> SADAQSFLNRVCGVSAARLTPCGTGTSTDVVYRAFDIYNDKVAGFAKFLKTNCCRFQEKDEDDNLIDSYFVVKRHTFSNYQHEETIYNLLKDCPAVAKHDFFKFRIDGDMVPHISRQRLTKYTMADLVYALRHFDEGNCDTLKEILVTYNCCDDDYFNKKDWYDFVENPDILRVYANLGERVRQALLKTVQFCDAMRNAGIVGVLTLDNQDLNGNWYDFGDFIQTTPGSGVPVVDSYYSLLMPILTLTRALTAESHVDTDLTKPYIKWDLLKYDFTEERLKLFDRYFKYWDQTYHPNCVNCLDDRCILHCANFNVLFSTVFPPTSFGPLVRKIFVDGVPFVVSTGYHFRELGVVHNQDVNLHSSRLSFKELLVYAADPAMHAASGNLLLDKR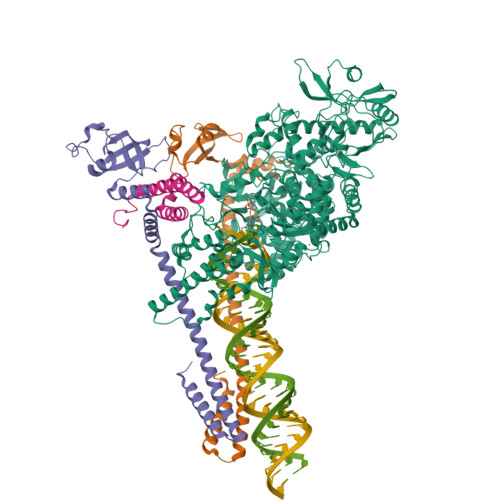TTCFSVAALTNNVAFQTVKPGNFNKDFYDFAVSKGFFKEGSSVELKHFFFAQDGNAAISDYDYYRYNLPTMCDIRQLLFVVEVVDKYFDCYDGGCINANQVIVNNLDKSAGFPFNKWGKARLYYDSMSYEDQDALFAYTKRNVIPTITQMNLKYAISAKNRARTVAGVSICSTMTNRQFHQKLLKSIAATRGATVVIGTSKFYGGWHNMLKTVYSDVENPHLMGWDYPKCDRAMPNMLRIMASLVLARKHTTCCSLSHRFYRLANECAQVLSEMVMCGGSLYVKPGGTSSGDATTAYANSVFNICQAVTANVNALLSTDGNKIADKYVRNLQHRLYECLYRNRDVDTDFVNEFYAYLRKHFSMMILSDDAVVCFNSTYASQGLVASIKNFKSVLYYQNNVFMSEAKCWTETDLTKGPHEFCSQHTMLVKQGDDYVYLPYPDPSRILGAGCFVDDIVKTDGTLMIERFVSLAIDAYPLTKHPNQEYADVFHLYLQYIRKLHDELTGHMLDMYSVMLTNDNTSRYWEPEFYEAMYTPHTVLQ;>[2x]AIASEFSSLPSYAAFATAQEAYEQAVANGDSEVVLKKLKKSLNVAKSEFDRDAAMQRKLEKMADQAMTQMYKQARSEDKRAKVTSAMQTMLFTMLRKLDNDALNNIINNARDGCVPLNIIPLTTAAKLMVVIPDYNTYKNTCDGTTFTYASALWEIQQVVDADSKIVQLSEISMDNSPNLAWPLIVTALRANSAVKLQ;> VACTKEVHMSKMSDVKCTSVVLLSVLQQLRVESSSKLWAQCVQLHNDILLAKDTTEAFEKMVSLLSVLLSMQGAVDINKLCEEMLDNRATLQ> GSQKERLLDELTLEGVARYMQSERCRRVICLVGAGISTSAGIPDFRSPSTGLYDNLEKYHLPYPEAIFEISYFKKHPEPFFALAKELYPGQFKPTICHYFMRLLKDKGLLLRCYTQNIDTLERIAGLEQEDLVEAHGTFYTSHCVSASCRHEYPLSWMKEKIFSEVTPKCEDC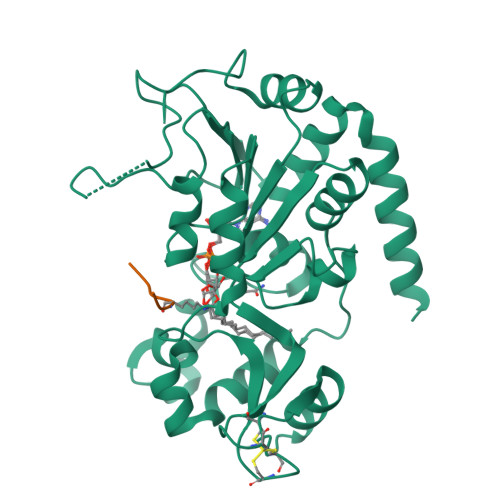QSLVKPDIVFFGESLPARFFSCMQSDFLKVDLLLVMGTSLQVQPFASLISKAPLSTPRLLINKEKAGQSDPFLGMIMGLGGGMDFDSKKAYRDVAWLGECDQGCLALAELLGWKKELEDLVRREHASIDAQ;> PRKQLA> MGSSHHHHHHMQFDV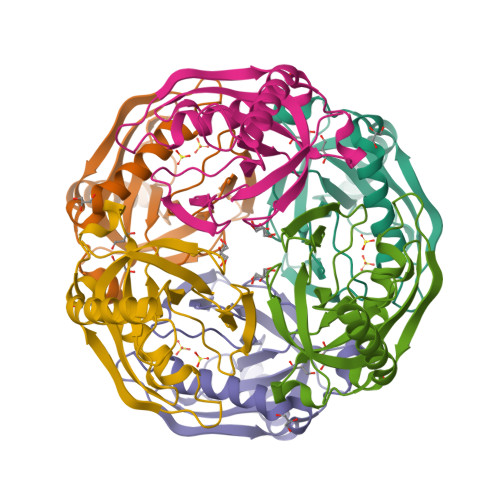TIEIPKGQRNKYEVDHETGRVRLDRYLYTPMAYPTDYGFIEDTLGDDGDPLDALVLLPQPVFPGVLVAARPVGMFRMVDEHGGDDKVLCVPAGDPRWDHVQDIGDVPAFELDAIKHFFVHYKDLEPGKFVKAADWVDRAEAEAEVQRSVERFKAGTH> MRVILNTGRTIWQGQAIESGKDLKMYVDAAAIIQMNPEMMKQLGIAEGDNVKVISEYGDVVVKAVEAKEPLPEGMVYIPMGPWANRVIRPYTDSTA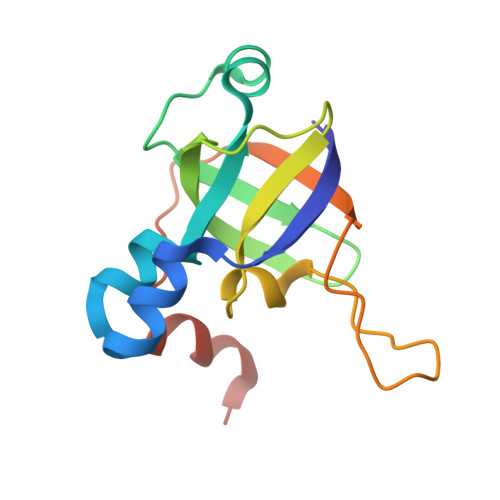TPSFKNIPVEIIPTDEEVLDMPTLMKVYGKVGQI>MEKLKLMTIVGTRPEIIRLSSTIKACDQYFNQILVHTGQNYDYTLNQIFFDDLELRQPDHYLEAVGSNLGETMGNIIAKTYDVLLREQPDALLILGDTNSCLAAVSAKRLKIPVFHMEAGNRCFDQNVPEEINRKIVDHVSDVNLPYTEHSRRYLLDEGFNKANIFVTGSPMTEVIEAHRDKINHSDVLNKLGLEPQQYILVSAHREENIDNEKNFKSLMNAINDIAKKYKMPVIYSTHPRSWKKIEESKFEFDPLVKQLKPFGFFDYNALQKDAFVVLSDSGTLSEESSILKFPGVLIRTSTERPEVLDKGTVIVGGITYNNLIQSVELAREMQNNNEPMIDAIDY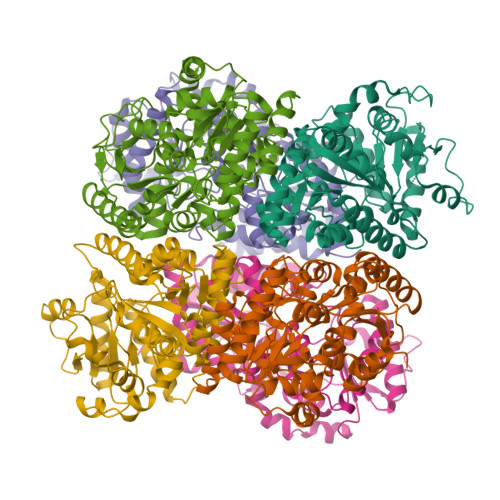KDTNVSTKVVKIIQSYKDIINRNTWRK[6x]Nuclear pore complex (NPC) is present in the nuclear envelope (NE) of all eukaryotic cells and mediates nucleocytoplasmic transport. A vertebrate NPC consists of four circular scaffolds: a cytoplasmic ring (CR), an inner ring (IR), a nuclear ring (NR), and a luminal ring (LR). IR resides in the central layer of the NPC and bridges the outer rings CR and NR. In this study, we report the cryo-EM reconstruction of the IR subunit of the X. laevis NPC at an average resolution of 4.2 Å, with local resolution reaching 3.8 Å.

We identified 30 molecules of nine distinct nucleoporins in each IR subunit, including four copies of Nup93, six copies of Nup155, four copies of channel nucleoporin hetero-trimer (CNT, each comprising Nup62/Nup58/Nup54),13 and two copies each for Nup205, Nup188, NDC1, and ALADIN. The IR subunit displays a 2-fold symmetry, with a cytoplasmic half and a nuclear half separated along the NE. At the center of the IR subunit, two molecules of Nup205 form a homo-dimer, which is flanked by two Nup188 molecules. Four molecules of Nup93 closely interact with the Nup205/Nup188 hetero-tetramer, with each Nup93 placing an extended helix into the axial groove of Nup205 or Nup188. The central scaffold associates with four CNTs on the side of the central pore of the NPC. All six Nup155 molecules in the IR subunit are located on the NE side, with their β-propellers directly contacting the NE. The elongated α-helical domains of Nup155-2 and Nup155-3 interact with each other in a roughly head-to-tail fashion, creating a homo-dimer of ~290 Å in length. The ALADIN–NDC1 hetero-dimer bridges the gap between Nup155-1 and Nup93-2 in the cytoplasmic half of the IR subunit. Notably, however, the spatial gap between these potentially interacting helices from S1 and S2 is large enough to disallow direct interactions. This analysis suggests a weak interface between neighboring IR subunits, which is consistent with the observed contraction and dilation of the NPC pore. However, the symmetric IR subunit is placed on the NE asymmetrically, tilting toward the cytoplasmic side by ~10°.

>[2x]MAAQLALNSEASLWGPYREIWQTVLSALIKRQPEAVHSLDIVLKKYKPDFISLFKNPPKSAQQHERVQKASTEGIPIKGTQRTRILEEQLIKEAFILSDLYNIGEIAAVELLLIGEQQQPTFHGLTRGLVAILLYWDGKSCMAESLLHLIQARKGKTFTLDHSPEVVSMVTRFTDDLMEQGLTNKILTLISQIDVNNEFDKLKKERGLGNKKHRKEVSDLIKECQQSLAHSLYSWSCQTPLNREDTLLLIGYLEKVTVEGDGSLDKVNLTLLMSLLYCLDVGFLEQGTDDREELMKQASMFMDRQYIAAIHNRLQNTQPWKSPGMQATVRLAWALALRGISQFSEVLEFSEADEPMAEIAIGGNVFLFLTEAVVGSESFCTDEFFIRRIHKLVTDFPTLMPMKVKQLRNRAEEDARLIQMSMQMGNEPPASLRRDLEHLLLLIGELYRKDPFHLELALEYWCPTEPLQSTSLMGSFLGVAHQRPPQRQVLLSKFVRQMSDLLPATLYLPYLKMLRGLASGPQCAHYCFSLLKANGGSSAENLQAAGGSPVSWDHFFHSLMLYHEHLRRDLPNTDNIHQRHPPLRGITQRELDGLIACLQLTCTIIDWSESARLALCEHAQWMPVVVILGLLQCSIPPLLKAELLKTLAAFGKSPEIAASLWQSLEYTQILQTVRATGLRQGVGIEVELNEIESRCEEYPLTRAFCQLISTLVESSFPTNLGAGLRAPGFEPYLQFLRDTVFLRYRTRAYRRAAEKWEVAEAVLDVFYKLLKDYEPQPEDFVDQYVELQGEERVAFKPPGFSLMHHLLNESPMLELCLSLMEEGVTQLDTYAPFPGKKHLEKAVAYCFMLLNLTLQKENRFMDLLRESHLSMIVTPLEQLLQGINPRSKKADNVVNIARYLCHGNSNAELAFESAKILCSISCNSKIQEKIVGDFTQDQNVSQKLMVGFVSCLDSEEAEELLDSEKEAEDQVKQTNIRYMTKIHILNLLITSLEMKAPNLAMFLLGYELKKPVSTTNLQDSGVLGCPRTCLHSILDILRKGTDVRAGPVAVWDTPHLAELCYQVIYQLCACADTSGPTMRYLRTSQDFLFSQLQHLPFSVEESEISAMNQMSWLMKTATIELRITSLNRQRSHTQRLLHLLLDDMPTRPYSADGEGGMEDESRSLSGFLHFDTTSKVRRKILRILDSIQFSNEIPEPLQLDFFDRSQIEQVIANCEHKNRRGQTVCNVKLLHRVLVAEVNALQGMAAIGQRPLLMEEINTILQYVVERNKLLQCLHAKRHALESWRQLVEIILTACPQDLIPTEHRQLIIRDLLQDLHVKILDDDAAQELMPIVAGAVFTLTAHLSQSVRTELKQPMTASGLGQSQYVQMLDGSFAAPPGTENISAGFASIGDSSLHMILRNLLEFILKTGGGFQRVRAHLYGSLLYYLQIAQRPDEPDTLESAHKSMWERLTAPEDVFSKLQRDNLSIFESYGTALMEVVCRDACDGHDIGRMLALALLDRIVSVDRQQQWLLYLSNSGYLKVLVDSLAEDDVVLRNLLTPQPPLLKALYIYESKMAFLTRVAKSSQGAIELLRSGVIVRLAQCQVYDMRPETDPHGVFGMRETPVFIPAPVERYRQILLPALQICQLILTSSTAQHLQAAGQVLQFLVAHSDTIQAILRSQEGSLGSLQELALLTGIISKAALPGVLNELDIGLNDGSMMELQGHIGRFQRQCLALLNRFGGSDRLRQLSLQDDSSRLDGVSKKDDMELAMQQICSNVMEYCQALMIQNSPSFQQTVCLFTPSLKESASRDGTRQDSQVSILPSWRLPSLGVVIHLLKQSANNFFTYYDIHRQSVGKLQNVEQLPPDEIKELCQSEMPVGADKISTTQKYGLARRRLVKLINSRAKLLSLCSYIIETCLYILWRHLEYYLLHCTTSDSQDPVFSNMTFGNRRFQDTFNTDPNMDPRNLRQNKVSQQDVDTLLREGANSFGESLQKRLLDIESLYCKVRSRHSFIQALVRRIRGLLRVSRV;>[2x]MAAAGSLYWRTSRELWTILLGRSSMKDGYQIKAELDRYGDRLLQGLAYYKPPSTRSADKVKANKNLSPALQELGLRLSKFLALDEEQSVELLQTYLQYDYRGTQESVKVLPQDERQSQALMLKMADYYYEERISLLRCVLYILNYFQDDKHPYSAEFSKCVELMEQKELFGKYLKQFESLCREEAPTWETHGNFMTERQVSRWFVQRLREQAMLLEIIFLYFACFAASPSDLLALTKLFKEQGFGCRLQNHHLVEPSMDPLVERIGYFSILIFLEALDMDTLMTCSLSDKIEQHPFSSEEQVCKEMDSILVTLGDVPHHGPVLLAWALLRFTLNPDKVTSAVRKMGSTAIQLHLFQYLTRMLQSLRSGENNCTTSTACLCVYTFLAYVLSTLEEQVSQSQQDLVETACQVFAAPNLPDLFWNMEPTAGLGILLDSVVGMFPFRISPLLKLFTALVSKSSAKKVYSFLDRMSSYTEHYRHKPHDILSHDDETLWKRQTPKLLYALGLGQTNLRIPQGALGQVMADENGFLVRWEYSYSCWTLFTCEIEMLLHVVSTADVIHQCQRVKPIIDLVHKVISTDLSIADCLLPITSRIYMLLQRLTTVMNPPMDFLSSCVDCLTALATRLPAKVWTDLRHTGFLPFAANPVSGHLISTEGMNAGGYGSLFGIEQSQGEYSVTLSFLRLITTLVKGQLGSTQSQGLVPCILFVLREMLPNYHRWRYNSHGVREQLGFQILSLIHAILNLCPEEEEGSSAPNLRSLCIFSLTNTEAGQAVINIMGIGVDTLNTVMLTQAGSSGTEGQGQMLMQTIKLAFSITNNVIRLKPPSSGVSPLEHALTQHGAHGNNLIAVLAKYIYHRYDPSLPRLAIQLLKRLAMVAPMSVYACLGSDAAAIRDAFLSRLRDNIEDMQIKIMILEFLTVAVETQPGLIELFLNLEAKDTNEGSKEYSLGEWSCLQVVLKLIDSQDPESSWGAPLLHRSAIAFLHALWQDRRDSAMTVLRTKPNFWENLTSPLFGTLACPSESSELSILETCAFIMKIICLEIYYAVRGSLGDSLKKILKKFSEEERFTYWSNYVHSLVCQVAETEGTCNSLTEYQQLLSAWRMFLIVATHNADVMHLTNPEVRQKLFKDILGGTQALLVVPRSVACMHLSSMLCTVMIILLRRWKNDLAAPEDILNSLTQILEGVLQRDQQLVEKTKAQIFSALISVLEMKPMKASEIPQYSQLLLNVCETLQEEVVSLVDHTRHEVPASDTSEDKDSMETEDTGRIRQKDQRDGVCVLGLHLAKELCEADEEGDQWQQVLRKLPVLPILFSALEVSLRIKQNLHFCEAILHFLFTLAKTHQGAAAMAGAGITQTVCLPLLSVYQLSSNGAGSVQPAVSLRKSLDAPSWPGVYRLTVSLMERLLKTLRYNFLSEALDFVGVHQERILQCLSAVRTVQSLSCLEEADHTVGFLLQLSNFTKEWHFHLPQLIKDVQVNLCYLCQACTSLLHSRKMLQHYLQIKNGESMSSTATPRGQRTPQTPSKQPTAESEALELRQLRTVQHSLLKILGKTLATLRAFTPDLCQILQVQPLDLAQYNLLFALSFTTPAFDADVTPSFGTLLATVNVTLSMLGEMDKKKDHPLSRALVESNNTGESKNNKSLLLFIMENCFYLLISQAVRYLRDPSVHPRDKQRMKQELSSELSTLLSSLSRYFRRGGPSSPAGGLMPSPQPKGASAAKVVPEAQEPLIQLVQAFVRHVQR;>[4x]MDGEGFGELLQQAEQLAAETEGVTELPHVERNLQEIQQAGERLRSKTMTRTSQESANVKASVLLGSRGLDISHISQRLESLSAATTFEPLEPVKDTDIQGFLKNEKDNALLSAIEESRKRTFVMAEEYHRESMLVEWEQVKQRVLHTLLASGEDALDFTQESETSYISESGAPGRSSLDNVEMAYARQMYMYNEKVVSGHLQPSLVDLCTEAAERLDDKNVSDLWVMVKQMTDVPLIPASDTLKSRCSGQMQMAFVRQALNYLEQSYKNYTLISVFANLQQAQLGGVPGTYNLVRSFLNIRLPTPIPGLQDGEIEGYPVWALIYYCMRCGDLMAAQQVVNRAQHQLGDFKNCFQEYIHNKDRRLSPTTENKLRLHYRRAVRASTDPYKRAVYCIIGRCDVSDNHSEVADKTEDYLWLKLSQVCFEDEANSSPQDRLTLPQFQKQLFEDYGESHFAVNQQPYLYFQVLFLTAQFEAAIAFLFRLERTRCHAVHVALALFELKLLLKSTGQSAQLLSQEPGEPQGVRRLNFIRLLMLYTRKFEPTDPREALQYFYFLRNEKDNQGESMFLRCVSELVIESREFDMLLGKLEKDGSRKPGAIDKFTRDTKTIINKVASVAENKGLFEEAAKLYDLAKNPDKVLELTNKLLSPVVSQISAPQSNRERLKNMALAIAERYKSQGVSAEKSINSTFYLLLDLITFFDEYHAGHIDLSFDVIERLKLVPLSQDSVEERVAAFRNFSDEIRHNLSEILLATMNILFTQYKRLKGSGPTTLGRPQRVQEDKDSVLRSQARALITFAGMIPYRMSGDTNARLVQMEVLMN;>MPSATPGAPAASAAMQEALEGAGRIIDRLLQEDRAYPDLSELLNVPVHTCPTISGVSEMDYPLQSPGLLTIPSLPEISAIRRVPLPPELIEQFGHMQCNCMMGVFPEISRAWLTIDSDIFMWNYEDGGDLAYYDGLSETILSVGLVKPKTGIFQPHIRFLLVLSTPVDIVILGLSFANLQPGNLNDSISGGMQLLPDPLYSLPTDNTYLLSITSTDNGRIFLSGKDGCLYEVEYQAEAGWFSQRCRKINHSKSSLSFLVPSVLQFAFSEDDPIVQIAIDNSRNILYTRSEKGVIQVYDLGVDGHGMSRVASVSQNSLVSAAGNIARTIDRNVFKPIIHISVIEMSESVNCHLLAVTHTGVRFYFSTVPFKQPTARPCMLALVHVRLPPGFSASSNVEKPSKVHKALYNNGVLLMAASENEDNDMLWCINRDSFPFQKPMMETQVTTQVDGHSWALSAVDEQKADKIVTPLNKDLIPLTDSPVIIQQHMIPPKRFVLLSAQGSHIFYKLRPVDQLRHLLVSNSGGDGEEIERFFKLHQENQACATCLILACSSAASDREVSSWAARAFFRYGGEAQLRVQSALHAPSNVGPIFGSPLPVASPIPVGSPMPNPSFLGTPTQGACPPNVSTPAYGVATPAPQPPAVPGMMGTEIVFSGKHNGICIYFCRIIGNIWDGSVAVENTFQSGNREVTAIDSSVTPQHLESVLKELKGLLEFLDRYSQFTAGSLGNPGFGTPANRQQRLVSLGRPDIGSSQQAQQELQRKYHTEAQLAEQFSLQGIHQLVRKMCQALALWKLLCEHQFSLVVSDLQKELQEQLKITTFKDLVIRDKELTGALTASLISCYIRDNASVDGISYRLQEVCPLLYSTDDAVCSKANELLQRSRHVPNKQEKERMLRESLKEYQKISQQVDLPNVCAQYRQVRFYEGVVELCLSAAEKKDPQGLGLHFHKNGEPEEDMAGLQAFQERLNSYKCITDTLQELVNQSKAAPQSPSVPKKPGPPVLSSDPNMLSNEEAGIHFEQMLKLAQRSADELFNIALFNWLIQADLTDKLLELNSPFLEPHLVRMAKLDQNKVRYMDLLWRYYEKNRNFSNAARVVAKLADMHSPEISLKQRLEYISRAILSAKSSTTMSTLAADGEFLHELEEKLEVARIQLQIQETLTRQYSHHSTVGDAVSQLDSQLMDITKMFGQYADPFRLSECKLAIIHCAGHSDPILVQTLWQDIIDKELSDSMGNSSVDRMQSLHLKITSLGKIYASTPRYFPLEFLVKYLEQQVCNFSWDAGFVTYTMQEINVPVPKLLEVYDHLFKARDPWWSRMKKPLHLLESIYILLSGYVQEPSKVPSYERRRFTTLCLDAISCYLVELQSMDPAPALLNTVSNFKSLQAKLERLS[6x];>MAFNFGATTGTPANQGTTGFSLGTFTPKTTTSGFGFGTTTTTAPTGFGGGFGGFGATTTASTGPAFSFTTPANTTSGLFGATQNKGFGFGTGFGSTTTSTGLGTGLGTGLGFTGFNTSQQQQQQSVLGAGLFNQSFQSTPQSNQLINTASALSAPTLLGDERDAILAKWNQLQAFWGTGKGFFMNNTPPVEFTQENPFCRFKAVGFSYIPNNKDEDGLISLIFNKKESDIRGQQQQLVESLHKVLGGHQTLTVNVEGVKTKADNQTEVIIYVVERSPNGTSRRVGASALFSYFEQAHIKANMQQLGVTGAMAQTELSPVQIKQLIQNPLSGVDPIIWEQAKVDNPDPERLIPVPMIGFKELLRRLEVQDQMTKQHQSRLDIISEDIGELQKNQTTTMAKIGQYKRKLMELSHRVLQVLIKQEIQRKSGFAIQAEEEQLRVQLDTIQSELNAPTQFKGRLNELMSQIRMQNHFGAVRSEEKYYVDADLLREIKQHLKQQQEGVSHLISIIKDNHEDIKLIEQGLNDNLHMRTGFLS[4x];>[4x]MSGFNFGAASAGGFSFGNPKSTTTTAPTGFSFGAATAAPSGGFSFGTATPTPASTTGQTSGLFSFSNPAPSLAPTSGFSFGAQVTSTPAPSSGGLAFGANTSKLNSGVGNQPAGGTTQTSQPMGGFSFGAATTQTQPSATSVGGFSFAGGVGSTSTNVFAQPAASTGITLQSAVSTAAAPTATTSQPTSTFSFGTQPQAAPALNFGLLSSSSVLSTASTPAAAQPVAPTTGLSLNFGKPADTSAAVTSTGSTTTNTPSLSSLLGTSGPSLFSSVATSTVPSVVSTVASGLSLTSTATSTGFGMKTLASSAVPTGTLATSTASLGVKAPLAGTIVQANAVGSAAATGISTATAMTYAQLENLINKWSLELEDQEKHFLQQATQVNAWDRTLMQNGERITTLHREMEKVKLDQKRLDQELDFILSQQKELEDLLTPLEESVKEQSGTIYLQHADEEREKTYKLAENIDAQLKRMAQDLKEVIEHLNTSAGPGDASNPLQQICKILNAHMDSLQWIDQNSALLQRKVEQVTKECESRRKEQERGFSIAFD;>MASGFSFGTAAASTTTLNPTAAAPFSFGATPAASNTGTTGGLGFGAFNAAATPATTTATTGLGGGLFGAKPAAGFTLGGANTATATTTAASTGFSVGFNKPAGSATPFSLPVTSTSSGGLSLASALTSTPATGPSPFTLNLGSTPATTTAAATGLSLGGTLTGLGGSLFQNTNPSATGLGQSTLGQSTLGQSTLGQSLLGQSLLGQSLLGQSTLGQSTLGQSLLGQSLLGLGLNLGAVAPVSQVTTHEGLGGLDFSSSSDKKSDKAGTRPEDSKALKDENLPQLLCQDVENFQKFVKEQKQVQEEISRMSSKAMLKVQEDIKALKQLLSVASSGLQRNALAIDKLKIETAEELKNAEIALRTQKTPPGLQHENTAPADYFHTLVQQFEVQLQQYRQQIEELENHLATQSNTLHLSPQDLSMAMQKLYQTFVALAAQLQAVNENFKMLKEQYLGYRKAFLGDSTDVFEARRAEAKKWQNAPRVTTGPTPFSNIPNAAAVAMAATLTQQQQPTTGFGSSSAFGGNTSGSSSFGFGTANKPSGSLSAGFGSTSTSGFNFSNPGINASAGLTFGVSNPSSTSFGTGQLLQLKKPPAGNKRGKR[4x];>MTMLGERLVLRWRVAASFAWSVILMPVCCALFIVLSRIQILHPIQWLTDSISDLTSSYTIFCLLLICAILGLQCTFLMEYYTVVPSIPCSRLALIGNLLLPHRILHSLAHVAMGVLASWCYAVLSKGKYQLLVVSCTLQSEDEADKPSHCLNESHLFQLLCGAFFGYSYSLQYFVHNMNYLSFPSIQQYKYLQFRRFLPLIIKQSVFQSLYFIRSYAILYFCLGNIPRTWIQTALNLHMDRQQPSLDTLRGFLNLSLFYQIWLSGTFLLATWYMVWILFRIYTTEARIFPVQTSFAEEAEKCLPFILNSNTLPLVKYLAMQDLVLLSQYSPSRRQEVFSLSQPGGHPHNWTSISKECLNLMSSLTSRLIAHQEAAANNGRMRVPSSPKQIRKSSSSSGTSLIEDSAEQTQNLSTIPRIGIPSLLKTASLKSSLDIGSPFATPGVKQMSESLDPNTPCHGSVQSPQVTRRGAKLWTSDSDVQKNGSEVSPVMHRPVCNGAKQGILHTWFQHKLVQIKNVLSKRGLIMYLFSKHPEASSQDVFADAQIHIWALEALSHLVAASFSEDRMGVVQTSLSSVLAILLTLQEAVEKHFKLPHASSKPARNPGSLLDSSCKTLRFSLRAALKTAIYRITTTFGEHLHAVPVSSEHKKKLQQFLDFKE[2x];>[2x]MCSLDLFPPPLDGSQLPLYEFNNEIVAGKGFDNPPPTFQSELVNIPEPTIPVDALKAPGRMELSSKTAFIHQKESIWKRCLNAWHNVGLAGFLEEMSNSKEEVPPWLCHVTRCSLAVCRSVSSLHGSLFPHLTISPQMKSEDLTAEFSQALGWADCPLRAFAWHPHTYKFALALLDDSIRIYTAGSPTIPTLKHRLQKDVASLAWKPMCASVLAVACQSCVLVWHVDPTSLSTRPSSGCAQVLSHPGHSPVTSVCWSPKGGVLLSASPVDTAMLVWDVPTESCIPLQRVGGGGVTFLSWSPDGSKVLAATPSSVFRVWETQKWTCERWPTLQGRCQTGCWSPDGSRLLFAVKGESVIYSLCFSVSEGEAQAGVGGSQSATVVADVSEVVFTTHTGEIRVGGEIQSMCWDPSGERLAVLLKGNPEFEESQPVIAVFRTRNSPIFELLPCGFIHGRKGETPQLFQFHPGFNKGALLSQLWSSGRVNHFPFYFVNAQCPRFSPESIAVVPGNTISTANPRTLFTER>[2x]TPVIPVASPDPALVNNPVVAATEPSVVKIRSLAPRCQKVLEGTGFVISPDRVM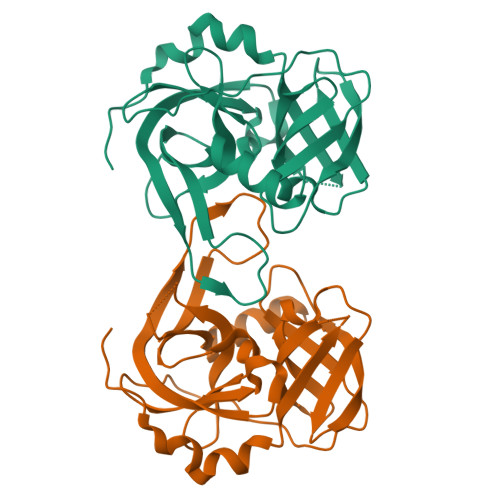TNAHVVAGSNNVTVYAGDKPFEATVVSYDPSVDVAILAVPHLPPPPLVFAAEPAKTGADVVVLGYPGGGNFTATPARIREAIRLSGPDIYGDPEPVTRDVYTIRADVEQGDSGGPLIDLNGQVLGVVFGAAIDDAETGFVLTAGEVAGQLAKIGATQPVGTGACVS(2S)-1-[4-[[(3R)-1,1-bis(oxidanylidene)thiolan-3-yl]methyl-methyl-amino]-6-methyl-pyrimidin-2-yl]-N-methyl-pyrrolidine-2-carboxamide 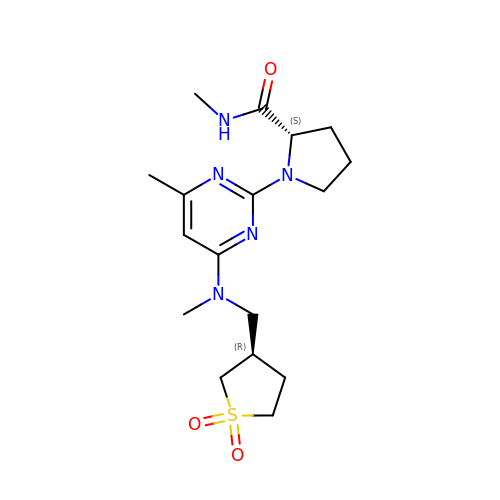| C17 H27 N5 O3 S | FPDVOQXTUVFQHW-KGLIPLIRSA-N>PMFIVNTNVPRASVPDGFLSELTQQLAQATGKPPQYIAVHVVPDQLMAFGGSSEPCALCSLHSIGKIGGAQNRSYSKLLCGLLAERLRISPDRVYINYADMNAANVGWNNS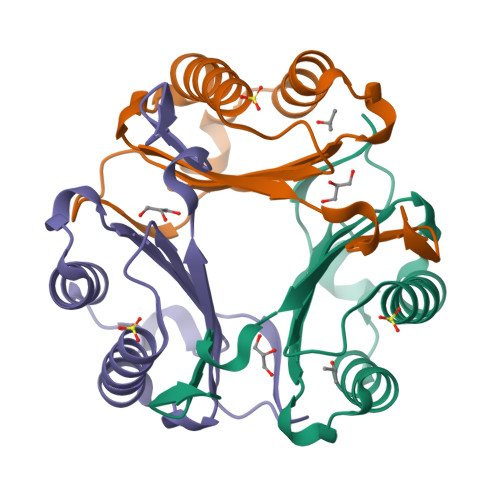TFA[3x]> MSYYHHHHHHLESTSLYKKAGLQALLLEQQDGKTLASVQTLDESRLPEGDVTVDVHWSSLNYKDALAITGKGKIIRNFPMIPGIDFAGTVRTSEDPRFHAGQEVLLTGWGVGENHWGGLAEQARVKGDWLVAMPQGLDARKAMIIGTAGFTAMLCVMALEDAGVRPQDGEIVVTGASGGVGSTAVALLH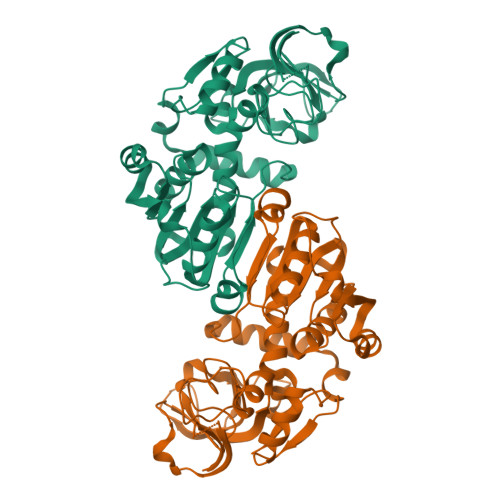KLGYQVVAVSGRESTHEYLKSLGASRVLPRDEFAESRPLEKQVWAGAIDTVGDKVLAKVLAQMNYGGCVAACGLAGGFTLPTTVMPFILRNVRLQGVDSVMTPPERRAQAWQRLVADLPESFYTQAAKEISLSEAPNFAEAIINNQIQGRTLVKVN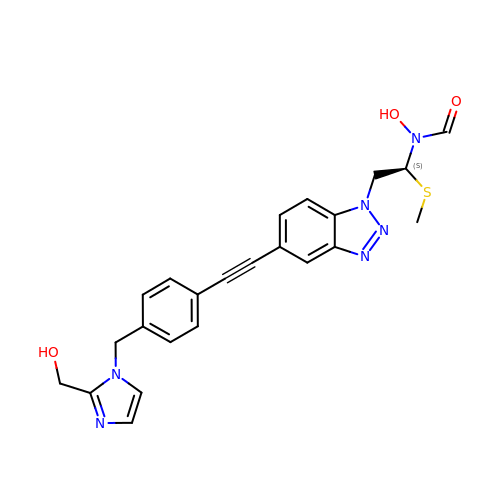N-hydroxy-N-[(1S)-2-{5-[(4-{[2-(hydroxymethyl)-1H-imidazol-1-yl]methyl}phenyl)ethynyl]-1H-benzotriazol-1-yl}-1-(methylsulfanyl)ethyl]formamide | C23 H22 N6 O3 S | PDKPBTURFVUWEE-QHCPKHFHSA-N>[4x]FVRKTNKNRDMPLDSDVFRVPPGYNAPQQVHITQGDLVGRAMIISWVTMDEPGSSAVRYWSEKNGRKRIAKGKMSTYRFFNYSSGFIHHTTIRKLKYNTKYYYEVGLRNTTRRFSFITPPQTGLDVPYTFGLIGDLGQSFDSNTTLSHYELSPKKGQTVLFVGDLSYADRYPNHDNVRWDTWGRFTERSVAYQPWIWTAGNHEIEFAPEINETEPFKPFSYRYHVPYEASQSTSPFWY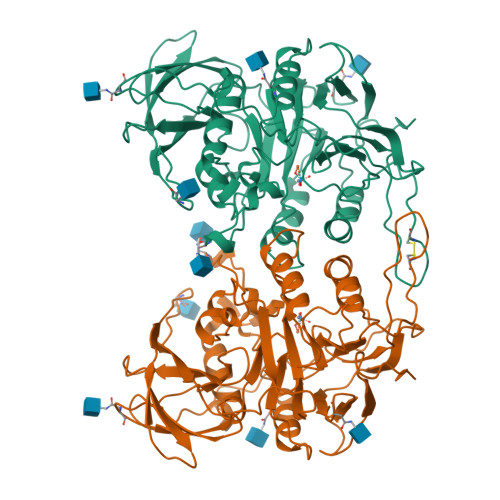SIKRASAHIIVLSSYSAYGRGTPQYTWLKKELRKVKRSETPWLIVLMHSPLYNSYNHHFMEGEAMRTKFEAWFVKYKVDVVFAGHVHAYERSERVSNIAYKITDGLCTPVKDQSAPVYITIGDAGNYGVIDSNMIQPQPEYSAFREASFGHGMFDIKNRTHAHFSWNRNQDGVAVEADSVWFFNRHWYPVDDST>MLEIKRYKNRVAARKSRAKFKQLLQHYREVAAAKSSENDRLRLLLKQMCP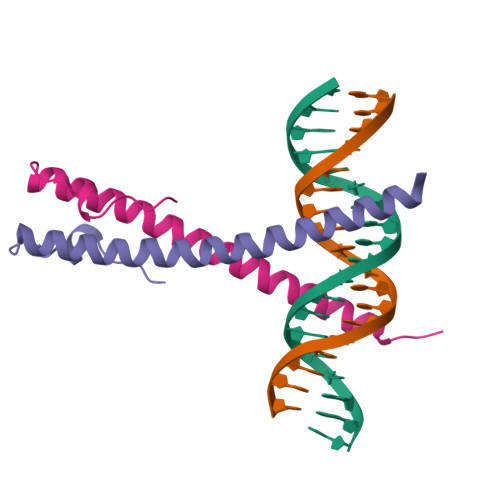SLDVDSIIPRTPD[2x]>[8x]HMNDMAHPNSAVLADFIPVQLAKPVPQRITLELTAYGFARAHCLSNGITDEEGFVQVYKTVKEKFDKYAVSPAQIKQRQLVYFPKLTDIRFGDGNFDIADPEPDQAHLRLFDIKKDPRGADLKTRHESYAKVVGKGLEQMFEGTLEAPDDLIHVTCSGYLAPSPAERMVADRGWFETTVTHSYNMGCYGA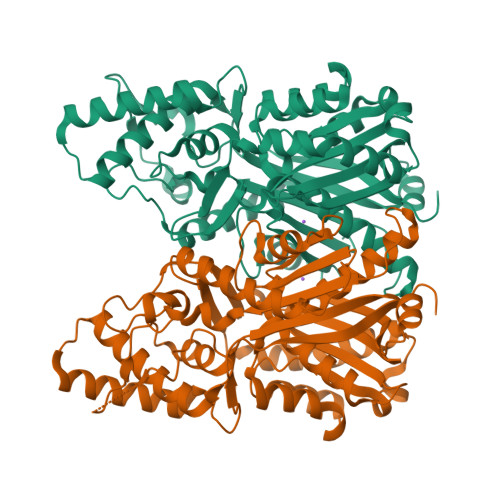FPAIKMAHGMLASAQWGATPPKTRVDIAHTELMSAHNNIAESRVDNIISATLFSDGLIKYSVYPEDELRRQGLRGLRILAMSEHLLPDSADTMTGVPGSHQFVMTLSPLVPAIIKRHVRAFAVDLLRRAGMDFERDKDALSFAIHPGGPKIVDHVQEELGLAEDQVAISKSVFLENGNMSSSTIPHILKAYLEEATVGTRIACLGFGPGLTAAGLVLEKI>PPKLCLVCSDEASGCHYGVLTCGSCKVFFKRAVEGQHNYLCAGRNDCIIDKIRRK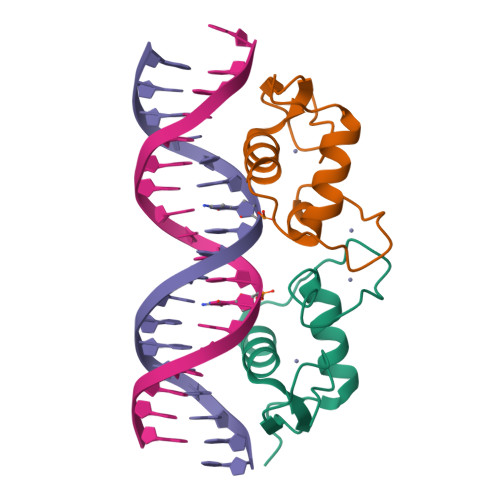NCPACRYRKCLQAGMNLEAR[2x]> MASN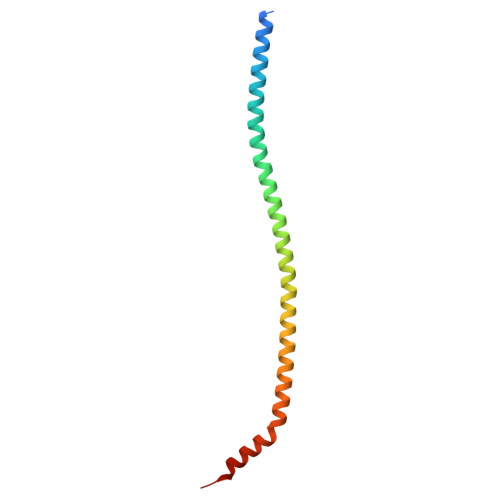RGHGGIQQLLAAEQEAQHIVAAARNAKMARLRQAKEEAEREIAEHRAQVEREFQRKLAESSGDSGANVKRLEQETEVKIHHLNAGAEKIQYDVVQMLLKHVTTVKN Here, inspired by natural and re-engineered protein–peptide systems, we set out to design proteins made out of repeating units that bind peptides with repeating sequences, with a one-to-one correspondence between the repeat units of the protein and those of the peptide. We use geometric hashing to identify protein backbones and peptide-docking arrangements that are compatible with bidentate hydrogen bonds between the side chains of the protein and the peptide backbone. We design repeat proteins to bind to six different tripeptide-repeat sequences in polyproline II conformations. The proteins are hyperstable and bind to four to six tandem repeats of their tripeptide targets with nanomolar to picomolar affinities in vitro and in living cells.

Reasoning that proline-containing peptides would incur a lower entropic cost upon binding than non-proline-containing peptides, we decided to start our experimental characterization with designs containing at least one proline residue; in most of these designs, the peptide backbone is in or near the polyproline II portion of the Ramachandran map. For the polyproline helix, there are roughly three residues per turn, and, probably because of this, we obtained more designs that target three-residue than two-residue proline-containing repeat units. Crystal structures reveal repeating interactions between protein and peptide interactions as designed, including ladders of hydrogen bonds from protein side chains to peptide backbones. Our results show that by matching superhelical parameters between repeating-protein and repeating-peptide conformations, and incorporating specific hydrogen-bonding and hydrophobic interactions between matched protein and peptide repeats, we can now design modular proteins that bind to extended peptides with high affinity and specificity.

> AWPAWPAWPAWP;> KKEAEEVAAHVEQIAFIAKEQGNEEVAKLAKRLAETIKRLNEGTEEEVKRLLEAAEVAAHVLQIAFIAHEQGNEEVAKLALELAESILRLIEGTEEEVKRLLEAAEVAAHVLQIAFIAHEQGNEEVAKLALELAESILRLIEGTEEEVKELLERAEEAAHVLQHAFIATEQGNEEDAKEALRKAEEILRRNA>[2x]AEKPKLHYFNARG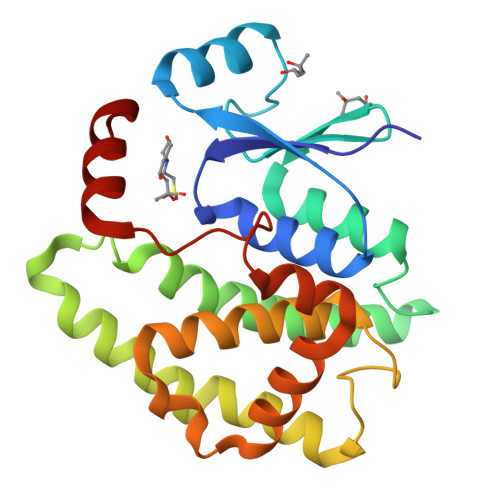RMESTRWLLAAAGVEFEEKFIKSAEDLDKLRNDGYLMFQQVPMVEIDGMKLVQTRAILNYIASKYNLYGKDIKERALIDMYIEGIADLGEMILLLPVCPPEEKDAKLALIKEKIKNRYFPAFEKVLKSHGQDYLVGNKLSRADIHLVELLYYVEELDSSLISSFPLLKALKTRISNLPTVKKFLQPGSPRKPPMDEKSLEEARKIFRF>[5x]MASLAAEPSDVFIGLKIDQITGINQKEENFSVVGSLRID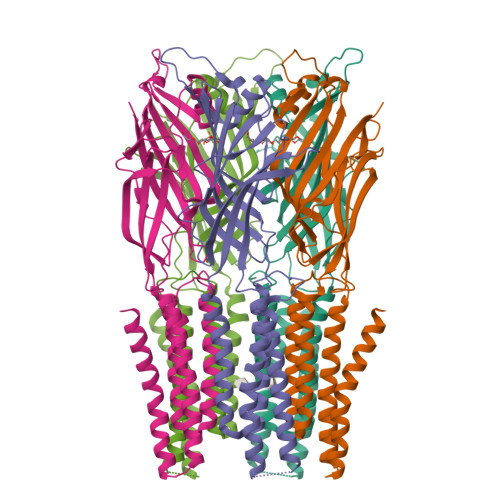WRQPLLAFEHAPGEPKHRTYTLATFLKLLEEKQIRWPAFTYHNQQGAMDFQNRLISLSEDGTVMYLERFTSTFQAPAFDFRLFPFDNQLFFIHVDSIFPQHLFRFQEMQGFSGLGDQLGEEEWIVTEVNTHLTTHNEFTKGDASRFVLEFHAERHLNYYLMRILIPVLLIITVSWFTFFLQDYTKRIDLAGGNLLLFIAFNFTISSDLPRLGYITLMDAFLVGTFIITALVVLGNVWLRRLENHGKQALARKLDIYAITSYPLAYLLGALTLWLLFFWRSY> MRNELEEMQRRADQLADESLESTRRMLQLVEESKDAGIRTLVMLDEQGEQL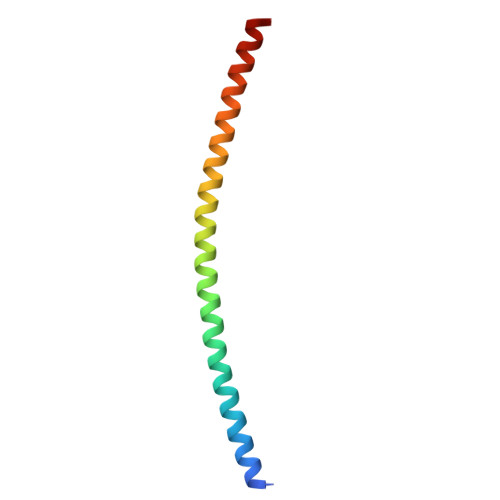DRVEEGMNHINQDMKEAEKNLKDLGK> GSHPFDQAVVKDPTASYVDVKARRTFLQSGQLDDRLKAA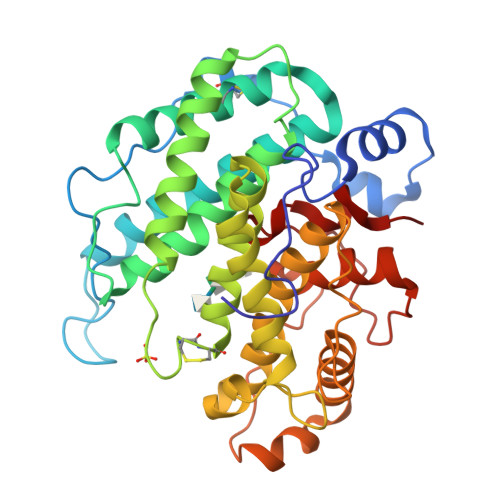LPKEYDCTTEATPNPQQGEMVIPRRYLSGNHGPVNPDYEPVVTLYRDFEKISATLGNLYVATGKPVYATCLLNMLDKWAKADALLNYDPKSQSWYQVEWSAATAAFALSTMMAEPNVDTAQRERVVKWLNRVARHQTSFPGGDTSCCNNHSYWRGQEATIIGVISKDDELFRWGLGRYVQAMGLINEDGSFVHEMTRHEQSLHYQNYAMLPLTMIAETASRQGIDLYAYKENGRDIHSARKFVFAAVKNPDLIKKYASEPQDTRAFKPGRGDLNWIEYQRARFGFADELGFMTVPIFDPRTGGSATLLAYKP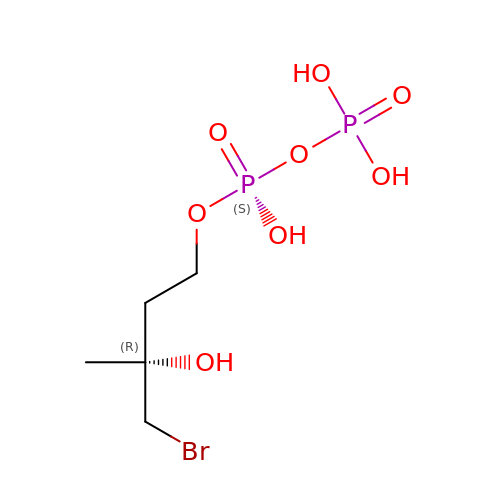4-BROMO-3-HYDROXY-3-METHYL BUTYL DIPHOSPHATE | C5 H13 Br O8 P2 | YKAYCWPQDPILSA-RXMQYKEDSA-N>GSSTNYGTIKWIFHALVFSYISFALISDKRYQKKEPLISSVHTKVKGIAEVKAEILENGMKKMVSGVFDTADYTFPLQGNSFFVMTNFIKTEGQQQGLCPDFPTARTICSSDRGCKKGRMDPQSKGIQTGRCVVYKERLKTCEVSAWCPIEEVKDAPRPALLNSAENFTVLIKNNIDFPGHNYTTRNILPGVNITCTFHKTQNPQCPIFRLGDIFQETGDSFSDVAIQGGIMGIEIYWDCNLDGWFHHCRPKYSFRRLDDKTTSESLYPGYNFRYAKYYKENNVEKRTLIKVFGIRFDILVFGTGGKFNVIQLAVYIGSVISYFGLATVFIDILINTYSASS[3x]

P2X receptors are the family of cation channels activated by extracellular ATP and are widely expressed in the mammalian nervous, respiratory, reproductive, and immune systems. There are seven subtypes (P2X1-P2X7) in the family, each of which plays distinct roles in physiological and pathophysiological functions via homo- or heterotrimerization. In this work, we determined the cryogenic electron microscopy (cryo-EM) structures of the panda P2X7 (pdP2X7) receptor in complex with PPADS and PPNDS. The overall structures are similar and show the trimeric architecture of P2X receptors, consisting of the extracellular domain and two transmembrane (TM) helices, with each protomer resembling the dolphin shape, consistent with the previously reported P2X structures (Sheng and Hattori, 2022).

The structures of pdP2X7 in the presence of PPNDS and PPADS were determined at 3.3 Å and 3.6 Å, respectively. In the PPNDS-bound and PPADS-bound structures, PPNDS and PPADS molecules bind to essentially the same orthosteric site, consistent with both PPNDS and PPADS being pyridoxal phosphate derivatives. It should be noted that while the pyridoxal phosphate groups in PPNDS and PPADS are shared, the naphthylazo group of PPNDS is significantly bulkier than the azophenyl group of PPADS. In both structures, the pyridoxal phosphate group has extensive interactions with the receptor. The phosphate group of PPNDS and PPADS interacts directly with the side chain of Arg294 and possibly also with Lys145, possibly via a water molecule. Furthermore, in the PPADS-bound structure, Lys64 mediates an additional interaction with the phosphate group. Interestingly, despite the structural differences between PPNDS and PPADS, the two common sulfonic acid groups form hydrogen bonds with the side chains of the same residues in the receptor, Lys66 and Gln143. In contrast, both PPNDS and PPADS possess only one phosphate group, so there was no corresponding downward movement in the left flipper domain. The binding of these competitive inhibitors may prevent the downward movement of the left flipper domain, which is required for channel opening. Consistent with antagonist binding, the TM domain adapts to the closed conformation of the channel, as similarly observed in the previously reported closed state structures of P2X7 receptors.>MKRKYLKLMIGLALAATLTLSGCSLPGLSAAADQTIKIGAQSMSESEIIASMLGQLIEHHTDLKTTTIKNLGSNAVQQQALMNGEIDIAATRYTGTALTGTLRMEPEKDPDKALALTQREFKKRYDLKWYDSYGFDNTYAFTVSKELADQYHLETVSDVKKWAPQLKLGVDNYWMKLKGNGYQDFTKTYGMTFGGTYPMQIGLVYDAVKSGKMDIVLAYSTDGRIKSYGLKMLKDDKQFFPPYDCSPVVPEKVLKEHPELEGIIKKMLGKIDTATMQELNYEVDGNLKEPSVVAKEYLEKH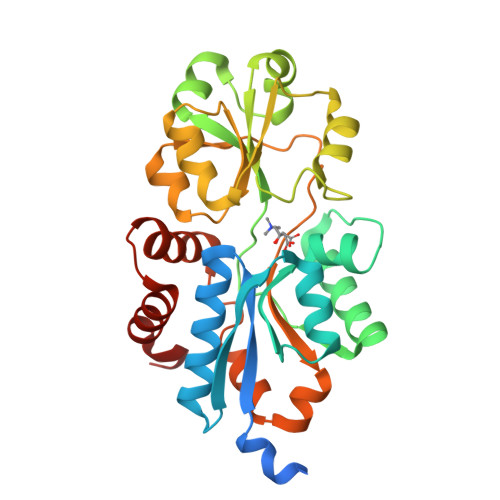RYFES[2x]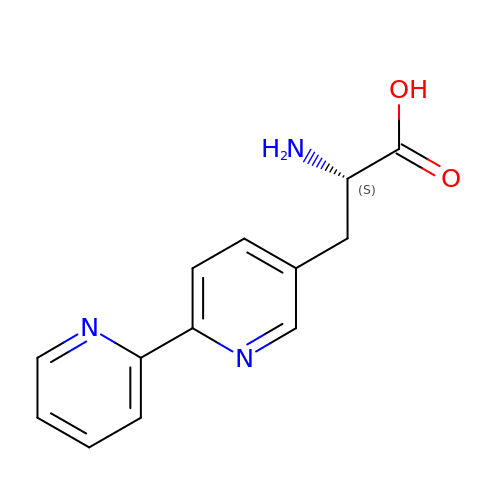3-(2,2'-BIPYRIDIN-5-YL)-L-ALANINE | C13 H13 N3 O2 | VWTQURBMIRJISI-JTQLQIEISA-N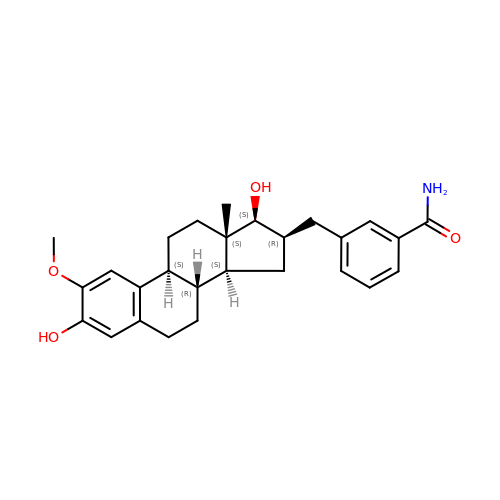3-{[(9beta,14beta,16alpha,17alpha)-3,17-dihydroxy-2-methoxyestra-1,3,5(10)-trien-16-yl]methyl}benzamide | C27 H33 N O4 | KFWAVTMEQBIVFP-YGIHYSQOSA-N IBANDRONATE | C9 H23 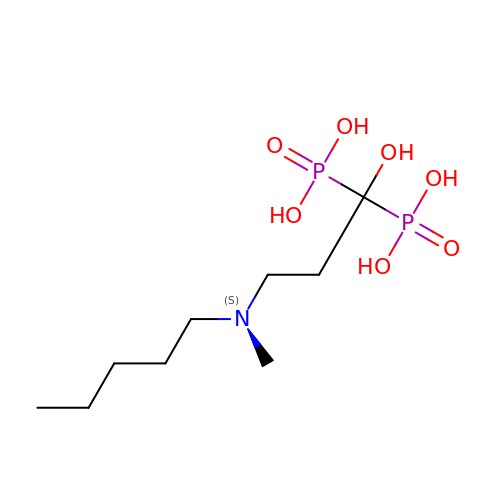N O7 P2 | MPBVHIBUJCELCL-UHFFFAOYSA-N>TNILAGAAVIKVLEAWGVDHLYGIPGGSINSIMDALSAERDRIHYIQVRHEEVGAMAAAADAKLTGKIGVCFGSAGPGGTHLMNGLYDAREDHVPVLALIGQFGTTGMNMDTFQEMNENPIYADVADYNVTAVNAATLPHVIDEAIRRAYAHQGVAVVQIPVDLPWQQIPAEDWYASANSYQTPLLPEPDVQAVTRLTQTLLAAERPLIYYGIGARKAGKELEQLSKTLKIPLMSTYPAKGIVADRYPAYLGSANRVAQKPANEALAQADVVLFVGNNYPFAEVSKAFKNTRYFLQIDIDPAKLGKRHKTDIAVLADAQKTLAAI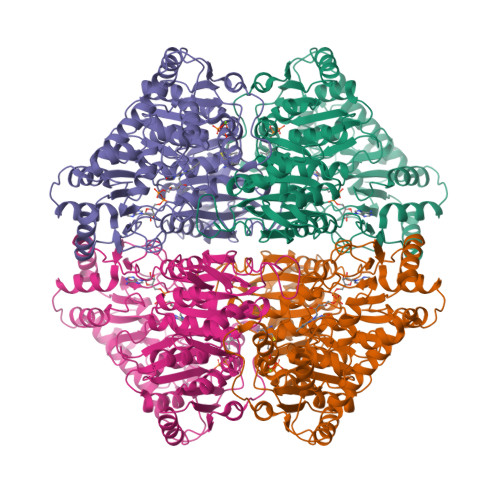LAQVSERESTPWWQANLANVKNWRAYLASLEDKQEGPLQAYQVLRAVNKIAEPDAIYSIDVGDINLNANRHLKLTPSNRHITSNLFATMGVGIPGAIAAKLNYPERQVFNLAGDGGASMTMQDLATQVQYHLPVINVVFTNCQYGFIKDEQEDTNQNDFIGVEFNDIDFSKIADGVHMQAFRVNKIEQLPDVFEQAKAIAQHEPVLIDAVITGDRPLPAEKLRLDSAMSSAADIEAFKQRYEAQDLQPLSTYLKQFGLDD[2x]> SNAMEHKIVHVGDIPVANDKPFTLFAGMNVLE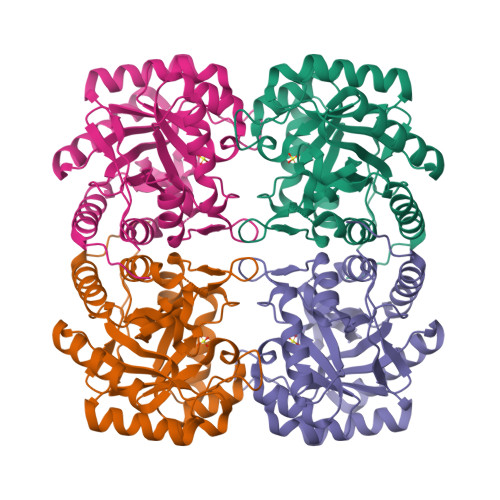SRDLAMQICEHYVKVTDKLGIPYVFKASFDKANRSSVHSYRGPGLEEGMKIFQELKETFGVKIITDVHTEAQAQPVADVVDVIQLPAFLARQTDLVEAMAKTGAVINVKKPQFMSPGQVGNIVEKFAECGNDKVILCERGSCHGYDNLVVDMLGFGVMKQASNGSPIIFDVTHSLQMRDPSGAASGGRREQTVELAKAGLATGIAGLFIEAHPNPDKARCDGPSALPLDKLEPFLAQMKALDDLIKSFAHIDIR> NLQNIIYNPVIPFVGTIPDQLDPGTLIVIRGHVPSDADRFQVDLQNGSSMKPRADVAFHFNPRFKRAGCIVCNTLINEKWGREEITYDTPFKREKSFEIVIMVLKDKFQVAVNGKHTLLYGHRIGPEKIDTLGIYGKVNIHSIGFSFS

Galectins are a family of proteins with some specificity for β-galactoside binding at their carbohydrate-recognition domain (CRD). Tandem-repeat-type galectins, like Gal-8, contain two distinct CRDs that are covalently connected via a peptide linker. In the present study, we used different conditions to crystallize the Gal-8 N-terminal CRD with its linker, and five structures could be solved. The N-terminal CRD prefers sulfated and sialylated glycans, whereas the C-terminal CRD prefers blood group A/B. In particular, the N-terminal CRD strongly binds to sulfated and sialylated glycans.

Our five structures were solved from crystals grown under two different conditions: (1) 20% (w/v) PEG2000 MME and (2) 0.1 M Tris pH 8.5, 0.01 M NiCl2, 20% (w/v) PEG2000 MME. Structures 1–3 were solved from the first condition and cryoprotectants for these three structures were glycerol, ethylglycol, and PEG400, respectively. Although the crystallization conditions were the same for structures 2 and 3, residues from the linker were less visible compared to our 1.08 Å structure. In structures 1–3, the N terminal tail (Gln9 to Ile12) forms a rigid loop, whereas in structures 4 and 5, the N terminal tail (Gln9 to Ile12) forms a small β-strand F0. In contrast in structures 1 to 3, no divalent caution was observed at this position. The resolution of C2 structures (structures 2 and 3, cryo-protected by ethylene glycol and PEG400, respectively) are lower than our P212121 structure (structure 1, cryo-protected by glycerol). The Rfree values of the C2 structures are higher than our P212121 structure, especially the Rfree value of the PEG400 structure. This indicates that cryoprotectants do play a role in determining the quality of Gal-8 N crystal structures.> SPSAEACGYSDRVLQLKLGNSAIVTQEAANYCCAYGEWPNYLPDHEAVAIDKPTQPETATDRFYTLKSVKWETGSTGWWWKLPDALNNIGMFGQN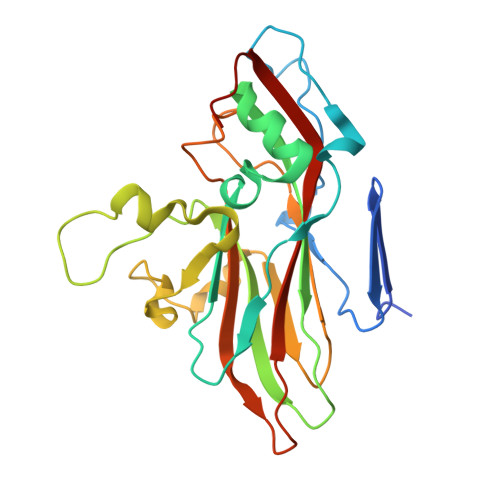VQHHYLYRSGFLIHVQCNATKFHQGALLVVAIPEHQRGAHNTNTSPGFDDIMKGEEGGTFNHPYVLDDGTSLACATIFPHQWINLRTNNSATIVLPWMNAAPMDFPLRHNQWTLAIIPVVPLGTRTTSSMVPITVSIAPMCCEFNGLRHAITQ>[6x]GSHMDLGFKSGIDLLKQRSTVWKLSTSSSELDSVLGGGLESQSVTEFAGVFGSGKTQIMHQSCVNLQNPEFLFYDEEAVSKGEVAQPKAVYIDTEGTFRPERIMQMAEHAGIDGQTVLDNTFVARAYNSDMQMLFAEKIED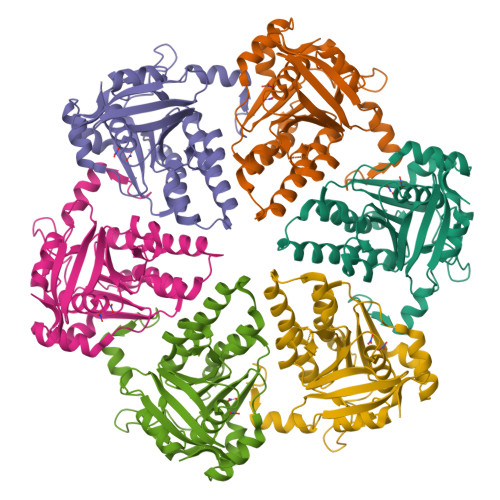LIQEGNNIKLVVIDSLTSTFRNEYTGRGKLAERQQKLGRHMATLNKLADLFNCVVLVTNQVSAKPDAFFGMAEQAIGGHIVGHAATFRFFVRKGKGDKRVAKLYDSPHLPDAEAIFRITEKGIQD> MTAIAPVI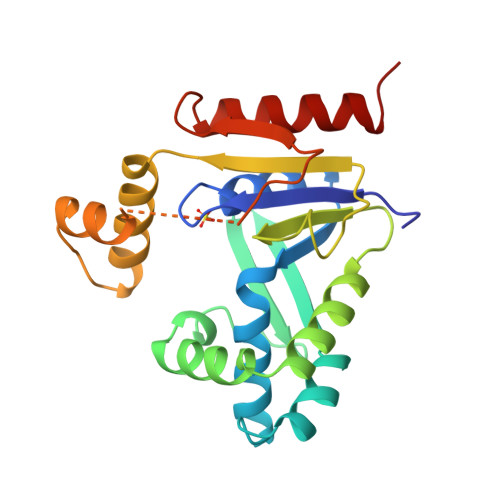TIDGPSGAGKGTLCKAMAEALQWHLLDSGAIYRVLALAALHHHVDVASEDALVPLASHLDVRFVSTNGNLEVILEGEDVSGEIRTQEVANAASQVAAFPRVREALLRRQRAFRELPGLIADGRDMGTVVFPDAPVKIFLDASSEERAHRRMLQLQVKGFSVNFERLLAEIKERDDRDRNRAVAPLVPAADALVLDSTTLSIEQVIEKALQYARQKLALA>SMSSLDINEQRALIKSAHRYISEKLEDHFSSEFLPKALVICGSGLSGISTKIADEPKPLILSYSTIPGFKVSTVPGHSGELIFGYMNGAPVV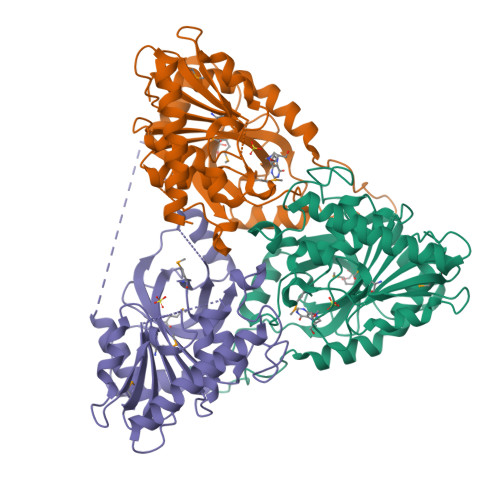LMNGRLHSYEGHSLAETVHPIRALHLLGSINVLIVTNAAGGINASFKAGDLMCVYDHINFPGLCGFHPLRGANFDEFGPRFLATSDAYDLELRKLLFSKKKELNIERKIHEGTYSYVHGPTFESRAESRFLRLAGTDAVGMSTVPEVVTARHCGWRVLALSLITNECVVDPPASAHDENPVPIQEGKATHEEVLENSAKASKDVQELIFSVVAEI[6x]> MATQMQQRDNGEETLANIKHSARSELKDMNVSGLAGINIQAGGYDLTGLSLTDELIAQGLSNVGLLPFEHSRVVLELAEAITVTANNTDMGGSGQYCEQGAWRAWLHVGLNMAKHHVRIRSSAAMDFGTHRMMACDPASLDASTISAMSRNVTTATMNAVSREMKAMKALAAGRSRMSQSDIADNNDCRGFAFGVLSRMVMHNSARRHGVVNGRLQELGENDASTADTYLTWELACAHGKGEVAITPVPAAWLDPEAQLTGRERVFSEALARLVDPDVGCVHVKIDGVTQNAAENARVHYATRPDPMSWLDDNTGLSADSNAGRISGEHYTLWKGRHSKVHLTIQLKQLYHRMSTTAATAEPRADSIVYYLKGFEGLGACAEFLLANSRFGHHSFLPGVFGVTADVHEAAYAQNQALFLAGIGDRMPPATFTKAQLATATYALMRRYDISERTCHFAITTIGHMVAQTAVRDLNNGSLSPLPFRVNLSPFLVQGVQFWDMNDTEGSVSVHDMGIGKELLTATYALGAMASLAHVCEQGGTGEEMSAIEVSRFTDVHTVATDLFRKVVMTELGDLKLRGSEVTHSSQEALFAQKMKAVWSSMAEGSTRLYNLNQAYGPFVDVQLARIRSSFVRDIGASRQMMDASALIKHAQNVTYDWPQNESGCPVQFIALPVPSTITHYATPAIGTERWFATTRLNAAGSKVISEIRWTNGLNSDDRAGVHVFAYGRSTIVSSPLGCAEAMAAMVIAGEHKVVRRHTSIARAQSARTANIVAGAVLGARNGDMMTIIRPSTSVASSAVHLRGYIPMAAMNMLPITDGDCDLVVADTRTRPGRMSTSPEAHRRGVLASDYHVDIATDGNIRHVAREVYTVADIPTVSERVSGLALRPYERSCVRDASTLHSMLCGAVPLLYGGGEPMKLGDNTPVTNRQALRPPEYNRNPALRMPARFQMGTTACAFTKALGDVRAQMELREGDVVTEEVTEPDTTIVPQGSITERVVVGEMTEALIMADQPMFDQDVVQNIMYNSPGIRGTERANIQAELMAAKDWPSILQATAKSSHGDIASAKTPYDLIKACKVDWSKVKGETQLKLIMNKIHPEYMTLSRAISAQVDARIVPNVPKSAMSTLLFWACATDMGLHTAVMANLAGLQRTTGFKGGIVYDLEGGANWPATDVRARIIEGWNAHARRIAQSGLISRDLTVMKIQHDMNADDIMALPAHIGDSWVLTIGELTANIATDEQSVAYAKDAQSAYYAIDRLRRLVAGREEGVDEILSKAEVMARVLAENKGLADDQALYHREWNRRTMAYVYMTTYLGSLDVEARLGVVSDDAYAERRAEWKAERAKLAVPAVSGQGQGRR;> MSAPSDQSQETRSPTSVGNTVAADVQTSVHDKPTGELKGSDGTGIHEATGLPIDKRGEVPTVQLERTAESIAKMMDLLRSEKFTAAAADAKLMLQQEFQNIVACAKNAPQMTVNAGRFYLGCNSTTAIIAGDTADGYEIEYSGKRIEGQCVVALEPLTITLSGSTSSTQDNSDSAKLFALAVSQVWGGASTVGIVAPMLQTVAQEQTFRARVERDSGFQHHAALTTVVTTIVGWLMHVGDSAAKRSRDGWLDHQTDFAVKGMLTPHIASGMDWAGVQTYSASAMETTTDRVRADYAGRMVVHSTLRKQTLRSRGTGDTTETENSGRYLLALPKCDAGVAAAALALTWGKPKLGGAGHANLTAVMSEAGVGYITGVNGTRATPHADTVFGREELVYLLGFALRHMADAQEQVIRNVLAQVASLFRPAACSAHEWMNVHGALMPKVSRPMNEPAFREVWNVANSSSDLQMIDRDKLNGEHFLRQLAQQITVNCTGTAMAIYQAVLAGPTGITDGDTTRLQKDLYHHLFQYATTTYADGVQVMQANTRMANKMVPPVNALAAWGLGSSMDSFTGPHCAYYFGLADAADGCFYSTTTGRTLSVYAVDVNHTSSDSYLAMAQLEPGLIATATGTGSTITTNVEAAGVVDGGLVTEGHVSLYTTISAQWNGLQREVYNWLLWHACKTEDSSHADIVGAEEVKSAVEWLSSNSVEAHRFRSSAGLGATEAAGSPGRRAWRLHHYDGQIFSNVIADTERHPYMRRLYTPSELRDARNDLFVVDRIWKIVMAMRAQLMLISVQEDGGRHQHSKHYFGEAAAIGVMGHGFTNLFAYCASTVHGGREARLISNCTDTPMYKKEANDLVPPMMKVAQLSTLLAHGGAWCNAVNMGGNSTSIGLSILGDGTMPLQTVPWTVNEITYLSEEGARHGIEAIIDTNGSVSVKVKMTMLEPRQRFCLYDDNKTSSYITAQESRTATYVTLKLGGTKNANTISGLVAHDYKLATTILASTYDKGRKTGLTLEDLQKVGGITGGQGMTGRGGGSSSGRGGRGRGGSSTGGAETIGDSE

We report the cryo-electron microscopy structure, at near-atomic resolution, of the double-stranded RNA Rosellinia necatrix quadrivirus 1 (RnQV1); this virus infects the fungus Rosellinia necatrix, a pathogenic ascomycete to a wide range of plants. At difference most dsRNA viruses, whose capsid is made of protein homodimers, RnQV1 is based on a single-shelled lattice built of 60 P2-P4 heterodimers. Despite a lack of sequence similarity, P2 and P4 have a similar α-helical domain, a structural signature shared with the dsRNA virus lineage. In addition to organizing the viral genome and replicative machinery, P2 and P4 have acquired new functions by inserting complex domains in preferential insertion sites.

Here we report the three-dimensional (3D) cryo-EM structure of the RnQV1 W1118 capsid at 3.7 Å resolution. The ~470 Å-diameter T = 1 capsid shows 12 outwardly protruding decamers at the pentameric positions (orange), each bearing five copies of P2 and P4. Each pentameric capsomer is formed by an inner ring of five P2 monomers (Fig 1D, blue; inset) surrounded by an outer ring of five partially intercalated P4 monomers (Fig 1D, yellow; inset), in which the asymmetric unit is a P2-P4 heterodimer. Our near-atomic models for P2 and P4 had 972 and 1005 residues, respectively, of the total 1356 (P2) and 1059 (P4) amino acids. P2 lacks 383 residues in the C-terminal region, predicted to have a high helical content, and P4 lacks 54 C-terminal residues. The structure of P2 (built from 29 α-helices and 20 β-strands) and P4 (29 α-helices, 9 β-strands) was organized similarly and was divided into two domains, a shell (S) and a protruding (P) domain (right). P2 and P4 overlapped considerably at the S domain. Both had a long α-helix tangential to the capsid surface, the α16 helix in P2 (36 Å long, 24 residues) and α15 in P4 (50 Å, 33 residues), a common characteristic of the dsRNA virus lineage CP (right, arrows). Analyses with Fatcat, Cath and Dali servers showed that this P2 domain has structural similarity, in addition to ferredoxin, to gelsolin and profilin, two actin-binding proteins with a variety of actin regulatory functions. The P4 Val648-His805 domain (in insertion site 2) has a surface cavity in which the last visible P2 C-terminal residue, Gly973, contacts P4 Ile791. We hypothesize that this surface crevice in P4 participates in proteolytic processing of the P2 C-terminal domain. In addition to the numerous weak interactions in the buried intra- and interdimeric surfaces that stabilize the capsid, there are five molecular hooks formed by short loops or α-helices that extend further on the rough contact surfaces, and contribute to pentamer stability (labeled I-V).(2R)-1-[(2R)-2-(2-methoxyethoxy)propoxy]propan-2-amine 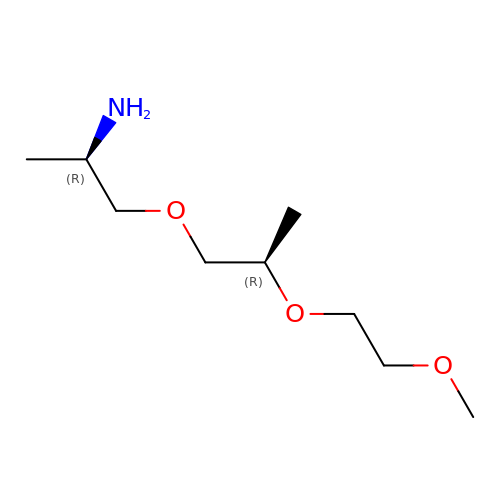| C9 H21 N O3 | QZWPAMVDKNPIHV-RKDXNWHRSA-N> MEDIIVVALYD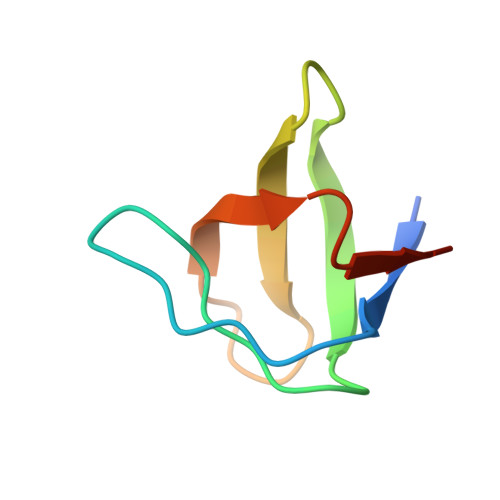YEGWWGDLSFQKGDQMVVLEESGEWWKARSLATRKEGYIPSNYVARVDS> SPPV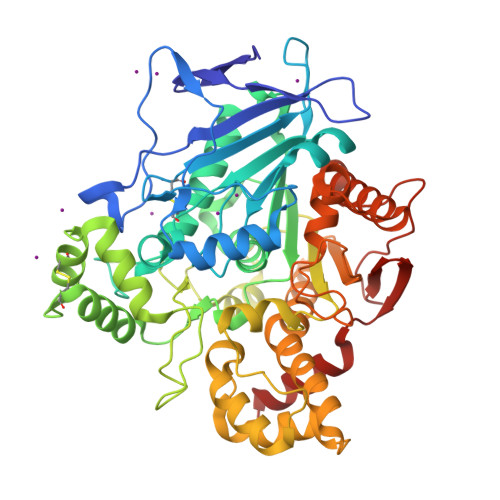VDTVHGKVLGKFVSLEGFAQPVAIFLGIPFAKPPLGPLRFTPPQPAEPWSFVKQATSYPPMCTQDPKAGQLLSELFTNRKENIPLKLSEDCLYLNIYTPADLTKKNRLPVMVWIHGGGLMVGAASTYDGLALAAHENVVVVTIQYRLGIWGFFSTGDEHSRGNWGHLDQVAALRWVQDNIASFGGNPGSVTIFGESAGGESVSVLVLSPLAKNLFHRAISESGVALTSVLVKKGDVKPLAEQIAITAGCKTTTSAVMVHCLRQKTEEELLETTLKMKFLSLDLQGDPRESQPLLGTVIDGMLLLKTPEELQAERNFHTVPYMVGINKQEFGWLIPMLMSYPLSEGQLDQKTAMSLLWKSYPLVCIAKELIPEATEKYLGGTDDTVKKKDLFLDLIADVMFGVPSVIVARNHRDAGAPTYMYEFQYRPSFSSDMKPKTVIGDHGDELFSVFGAPFLKEGASEEEIRLSKMVMKFWANFARNGNPNGEGLPHWPEYNQKEGYLQIGANTQAAQKLKDKEVAFWTNLFAK4-[6-amino-5-(3,5-difluoro-4-hydroxyphenyl)pyridin-3-yl]benzene-1-sulfonamide | C17 H13 F2 N3 O3 S | 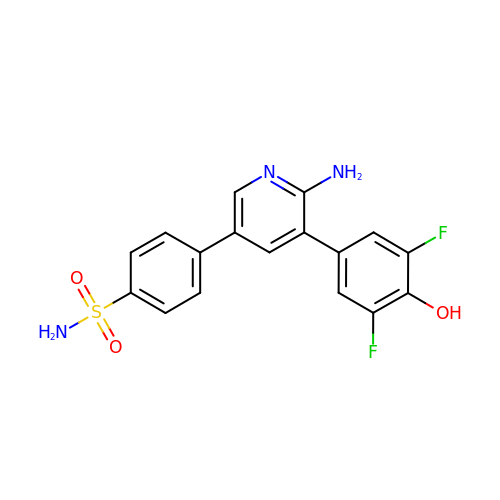MTBXQYCZMOAADV-UHFFFAOYSA-N>MGHHHHHHAMEGKITPVSVKKVDDKVTLYKTTATADSDKFKISQILTFNFIKDKSYDKDTLVLKATGNINSGFVKPNPNDYDFSKLYWGAKYNVSISSQSNDSVNVVDYAPKNQNEEFQVQNTLGYTFGGDISISNGLSGGLNGNTAFSETINYKQESYRTTLSRNTNYKNVGWGVEAHKIMNNGWGPYGRDSFHPTYGNELFLAGRQSSAYAGQNFIAQHQMPLLSRSNFNPEFLSVLSHRQDGAKKSKITVTYQREMDLYQIRWNGFYWAGANYKNFKTRTFKSTYEIDWENHKVKLLDTKETENNK[4x];>MGHHHHHHAMANDTEDIGKGSDIEIIKRTEDKTSNKWGVTQNIQFDFVKDKKYNKDALILKMQGFISSRTTYYNYKKTNHVKAMRWPFQ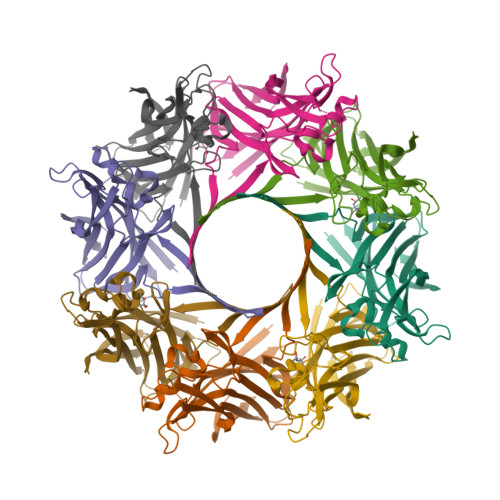YNIGLKTNDKYVSLINYLPKNKIESTNVSQTLGYNIGGNFQSAPSLGGNGSFNYSKSISYTQQNYVSEVEQQNSKSVLWGVKANSFATESGQKSAFDSDLFVGYKPHSKDPRDYFVPDSELPPLVQSGFNPSFIATVSHEKGSSDTSEFEITYGRNMDVTHAIKRSTHYGNSYLDGHRVHNAFVNRNYTVKYEVNWKTHEIKVKGQN[4x]> SGRPMSSMNPEYDYLFKLLLIGDSGVGKSCLLLRFADDTYTESYISTIGVDFKIRTIELDGKTIKLQIWDTAGQERFRTIT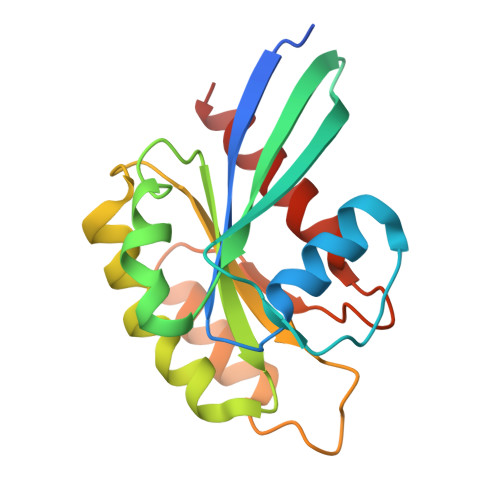SSYYRGAHGIIVVYDVTDQESFNNVKQWLQEIDRYASENVNKLLVGNKCDLTTKKVVDYTTAKEFADSLGIPFLETSAKNATNVEQSFMTMAAEIKKRMG2-heptyl-4,6-bis(oxidanyl)benzoic acid | C14 H20 O4 | 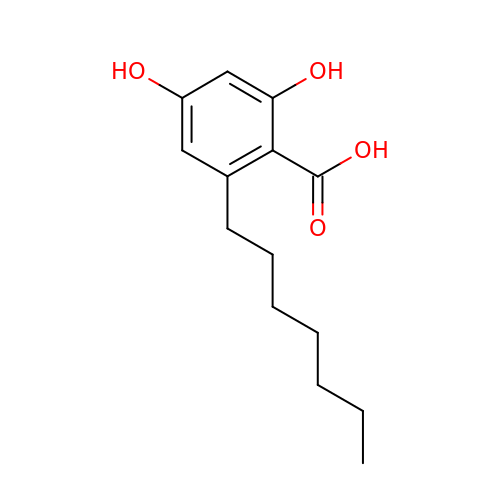XUWGCDWPOGIQII-UHFFFAOYSA-N> GPLVETRTIVRFNRPFLM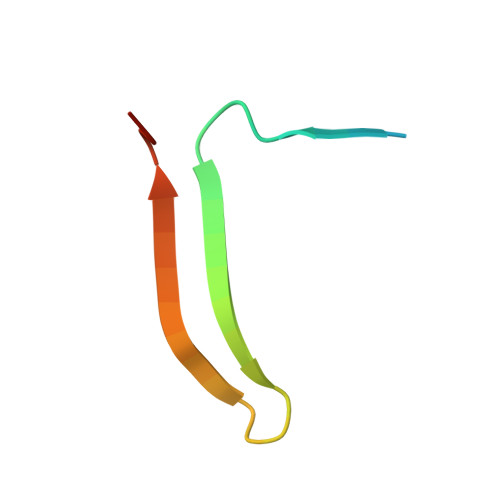IIVDHFTWSIFFMSKVTNPKQA> AGAGGUUCUAGCACAUCCCUC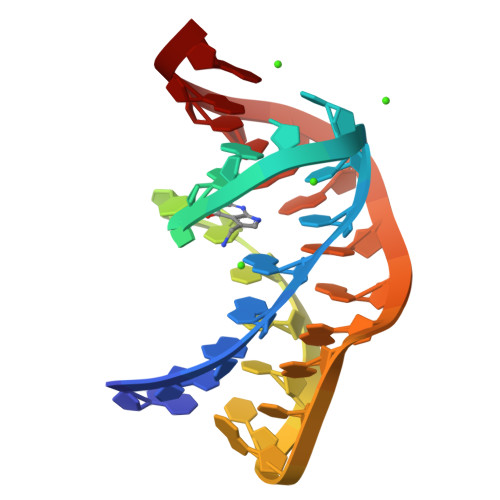UAUAAAAAACUAA>MKYAGILAGGIGSRMGNVPLPKQFLDLD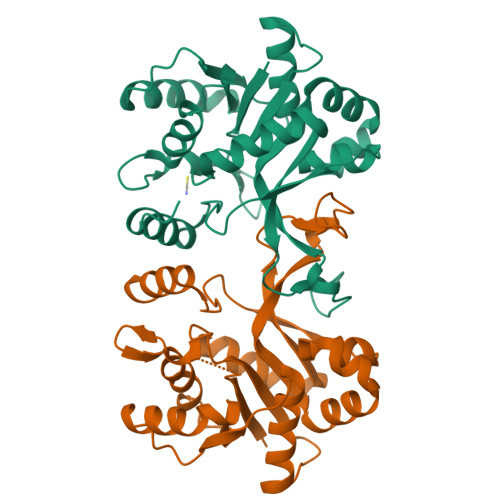NKPILIHTLEKFILINDFEKIIIATPQQWMTHTKDTLRKFKISDERIEVIQGGSDRNDTIMNIVKHIESTNGINDDDVIVTHDAVRPFLTHRIIKENIQAALEYGAVDTVIDAIDTIVTSKDNQTIDAIPVRNEMYQGQTPQSFNINLLKESYAQLSDEQKSILSDACKIIVETNKPVRLVKGELYNIKVTTPYDLKVANAIIRGGIADDGGSLVPRGSAAAALEHHHHHHHH[6x]> MG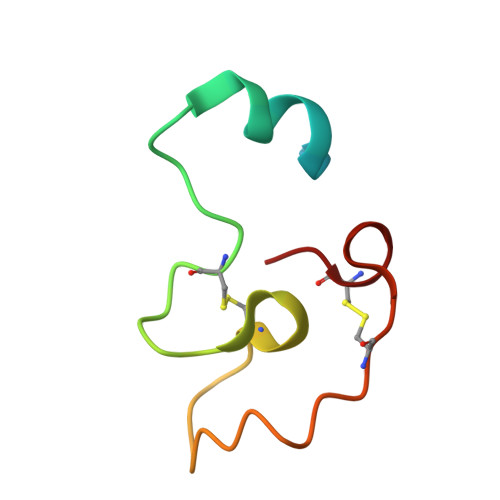RRQLARGRRYIGYDALKKNNVPCSRRGRSYYDCKKRRRNNPYRRGCSAITHCYR>GPDSMNFSPTKRVEKPQLKFKSPIDNSESHPFIPLLKEKPNALKPLSESLRLVDDDENNPSHYPHPYEYEIDHQEYSPEILQIREEIPSKSWDDSVPIWVDTSTELESMLEDLKNTKEIAVDLEHHDYRSYYGIVCLMQISTRERDYLVDTLKLRENLHILNEVFTNPSIVKVFHGAFMNIIWLQRDLGLYVVGLFDTYHASKAIGLPRHSLAYLLENFANFKTSKKYQLADWRIRPLSKPMTAYARADTHFLLNIYDQLRNKLIESNKLAGVLYESRNVAKRRFEYSKYRPLTPSSEVYSPIEKESPWKILMYQYNIPPEREVLVRELYQWRDLIARRDDESPRFVMPNQLLAALVA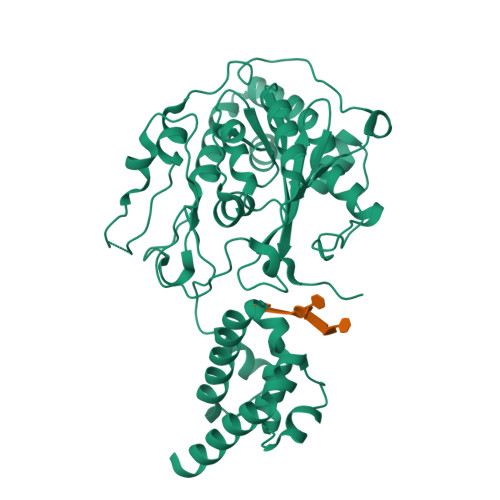YTPTDVIGVVSLTNGVTEHVRQNAKLLANLIRDALRNIKNTNEE[2x]>SMRKKIFKPEELRQALMPTLEALYRQDPESLPFRQPVDPQLLGIPDYFDIVKNPMDLSTIKRKLDTGQYQEPWQYVDDVWLMFNNAWLYNRKTSRVYKFCSKLAEVFEQEIDPVMQSLG[3x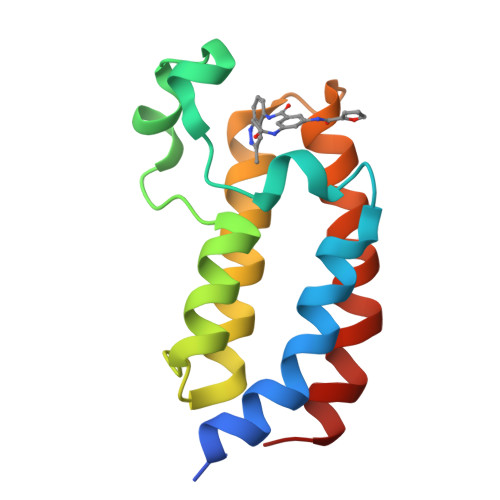]>[16x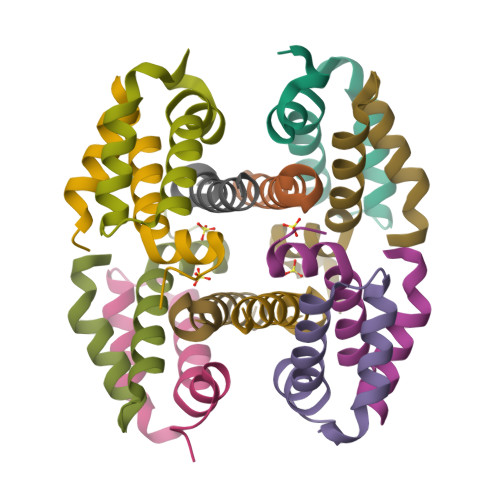]GKVDLQSLPTRAYLDQTVVPILLQGLAVLAKERPPNPIEFLASYLLKNKAQFEDRN;>GAMGSVEHTLADVLYHVETEVENLYFQ[8x]> MAEDADMRNE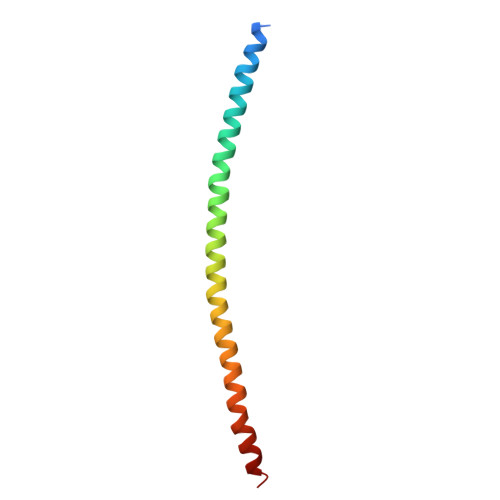LEEMQRRADQLADESLESTRRMLQLVEESKDAGIRTLVMLDEQGEQLDRVEEGMNHINQDMKEAEKNLKDLGK> MPPKARAPLPPGDVERGEKLFKGRAAQC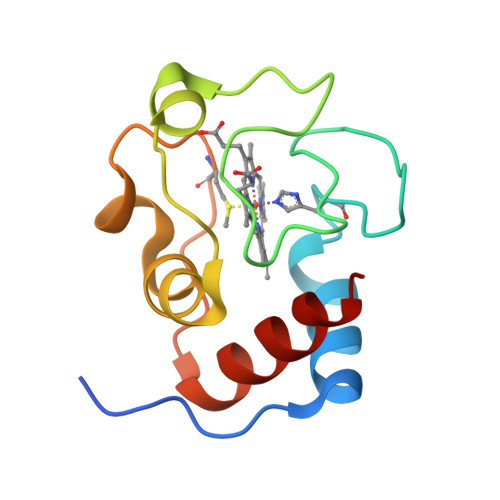HTATKGGSNGVGPNLFGIVNRPSGKVEGFTYSKANAESGVIWTPEVLDVYLENPKKFMPGTKMSFAGIKKPQERADVIAYLETLK> MKIVYWSGTGNTEKMAELIAKGIIESGKDVNTINVSDVNIDELLNEDILILGCSAMDDEVLEESEFEPFIEEISTKIS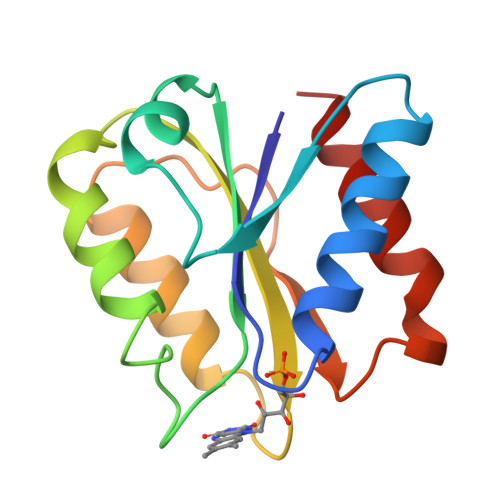GKKVALFGSYGWGDGKWMRDFEERMNGYGCVVVETPLIVQNEPDEAEQDCIEFGKKIANI> CGCGUCAC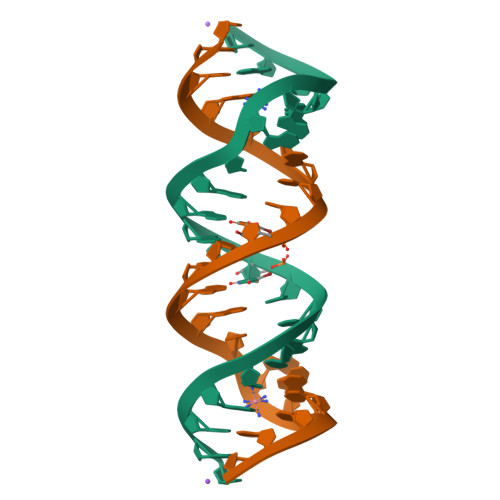CUCGAGCAAGUCGC> VTFDVGDEYEIIETIGNGAYGVVSSARRRLTGQQVAIKKIPNAFDVVTNAKRTLRELKILKHFKHDNIIAIKDILRPTVPYGEFKSVYVVLDLMESDLHQIIHSSQPLTLEHVRYFLYQLLRGLKYMHSAQVIHRDLKPSNLLVNENCELKIGDFGMARGLCTSPAEHQYFMTEYVATRWYRAPELMLSLHEYTQAIDLWSVGCIFGEMLARRQLFPGKNYVHQLQLIMMVLGTPSPAVIQAVGAERVRAYIQSLPPRQPVPWETVYPGADRQALSLLGRMLRFEPSARISAAAALRHPFLAKYHDPDDEPDCAPPFDFAFDREALTRERIKEAIVAEIEDFHARRE

The ERK5 protein, which is encoded by the MAPK7 gene, comprises an N-terminal kinase domain and a large C-terminal domain containing transcriptional transactivating functionality and nuclear localization and export sequences (NLS/NES). ERK5 is the effector kinase of a canonical kinase module comprising MEK (MAPK/ERK kinase) 5, MEKK (MEK kinase) 2/3 and ERK5 itself.

Compounds 2 and 3, like compound 1, bind at the conventional ATP-binding site, while compounds 4, 5 and 6 bind at a novel allosteric binding site. The allosteric binding site is located in a cleft between the P-loop and the αC helix adjacent to the ATP-binding site. An intramolecular hydrogen bond between the amide O atom and the aniline N atom forms a pseudo-bicyclic ring system that maintains the compound in a planar conformation. The primary amine donates hydrogen bonds to the side chains of both Asn95 and Thr99 from the αC helix. One face of the pocket is defined by the side chains of Arg98 and Glu102 from the αC helix, which form a favourable salt bridge with one another. π–π stacking is observed between the triazole ring and the guanidinium group of Arg98. Formation of a hydrogen bond between Glu102 and the hydroxyl group of Tyr66 from the tip of the P-loop stabilizes the P-loop in a closed conformation. The side chain of Lys84 is displaced by binding of compounds 4–6 and reorients to form a hydrogen bond to the backbone carbonyl of Val68 from the P-loop. Glu102, meanwhile, adopts an alternative rotamer allowing the formation of a salt bridge with Arg98 and a hydrogen bond to Tyr66. This new network of hydrogen bonds contributes to stabilization of the allosteric pocket. Differential flexibility in the P-loop amongst kinases has been implicated in the selectivity of certain conventional ATP-binding site-targeted kinase inhibitors, and may have implications for the selectivity of our allosteric ERK5 inhibitors (see §3.5). In contrast to the P-loop, the αC helix orientation is unchanged upon the binding of compounds 4–6.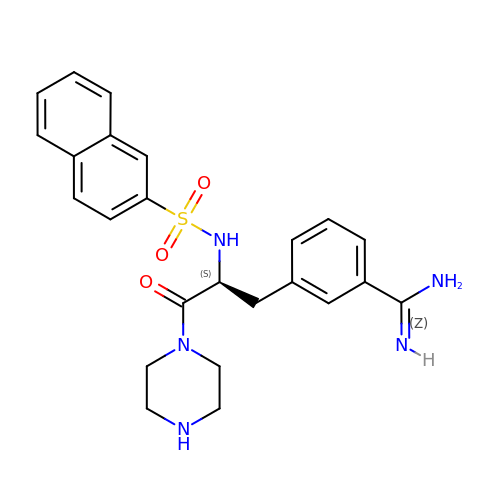N-ALPHA-(2-NAPHTHYLSULFONYL)-3-AMIDINO-L-PHENYLALANINE PIPERAZIDE | C24 H27 N5 O3 S | ZVDMTWWOKZXJOE-QFIPXVFZSA-N>[4x]MYRMDKYTIGLIRVITLEDKEILNLHGRIIESAFPELKVVSRCIEDQPKGIYNEETERE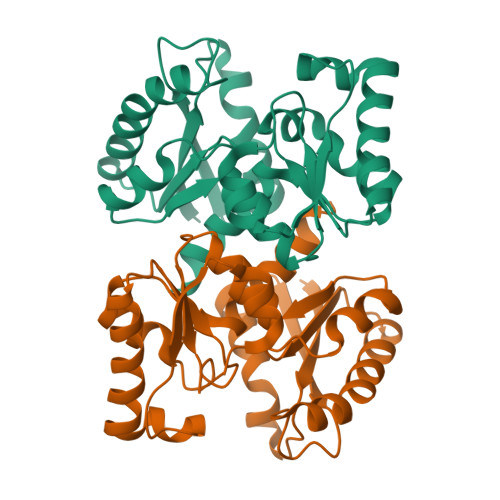AEPKIIRLAKEFEREGVDAIIISCAADPAVEKVRKLLSIPVIGAGSSVSALALAYGRRVGVLNLTEETPKVIRSILGNNLIAEDHPSGVSNTLDLLTDWGRREVINAAKRLKEKGVEVIALGCTGMSTIGIAPVLEEEVGIPVIDPVIASGAVALHALKRREVKRFEGR> MKN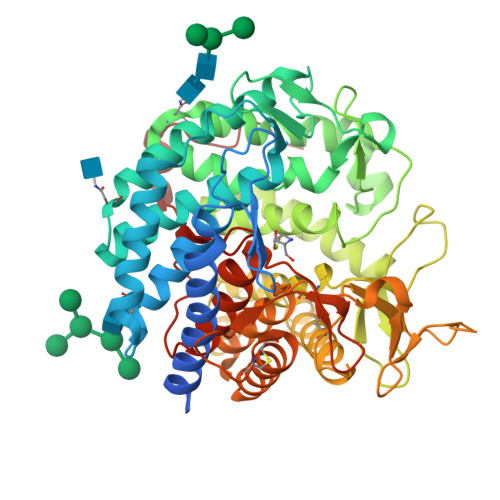SVGISIATIVAIIAAIYYVPWYEHFERKSPGAGEMDRDRIESMFLESWRDYSKHGWGYDVYGPIEHTSHNMPRGNQPLGWIIVDSVDTLMLMYNSSTLYKSEFEAEIQRSEHWINDVLDFDIDAEVNVFETTIRMLGGLLSAYHLSDVLEVGNKTVYLNKAIDLGDRLALAFLSTQTGIPYSSINLHSGQAVKNHADGGASSTAEFTTLQMEFKYLAYLTGNRTYWELVERVYEPLYKNNDLLNTYDGLVPIYTFPDTGKFGASTIRFGSRGDSFYEYLLKQYLLTHETLYYDLYRKSMEGMKKHLLAQSKPSSLWYIGEREQGLQGQLSPKMDHLVCFMGGLLASGSTEGLSIHEARRRPFFSKSDWDLAKGITDTCYQMYKQSSSGLAPEIVVFNDGNIKQDGWWRSSVGDFFVKPLDRHNLQRPETVESIMFMYHLSHDHKYREWGAEIATSFFENTCVDCNDPKLRRFTSLSDCITLPTKKSNNMESFWLAETLKYLYILFLDEFDLTKVVFNTEAHPFPVLDEEILKSQSLTTGWSL> SMPDGCYADGTWELSVHVTDLNRDVTLRVTGEVHIGGVMLKLVEKLDVKKDWSDHALWWEKKRTWLLKTHWTLDKYGIQADAKLQFTPQHKLLRLQLPNMKYVKVKV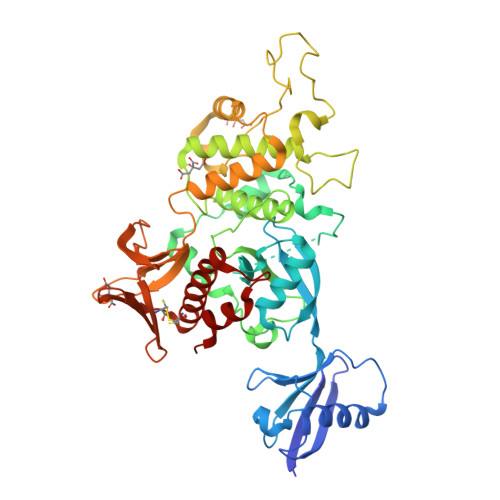NFSDRVFKAVSDICKTFNIRHPEELSLLKKPRDPTKKKKKKLDDQSEDEALELEPGILAVSQPITSPEILAKMFKPQALLDKAKINQGWLDSSRSLMEQDVKENEALLLRFKYYSFFDLNPKYDAIRINQLYEQAKWAILLEEIECTEEEMMMFAALQYHINKLSIMTSENHLNNSDKEVDEVDAALSDLEITLEGGKTSTILTTDITPECLVSPRYLKKYKNKQITARILEAHQNVAQMSLIEAKMRFIQAWQSLPEFGITHFIARFQGGKKEELIGIAYNRLIRMDASTGDAIKTWRFSNMKQWNVNWEIKMVTVEFADEVRLSFICTEVDCKVVHEFIGGYIFLSTRAKDQNESLDEEMFYKLTSGWV> SNAADPEVCCFITKILCAHGGRMALDALLQEIALSEPQLCEVLQVAGPDRFVVLETGGEAGITRSVVATTRARVCRRKYCQRPCDNLHLCKLNLLGRCNYSQSERNLCKYSHEVLSEENFKVLKNHELSGLNKEELAVLLLQSDPFFMPEICKSYKGE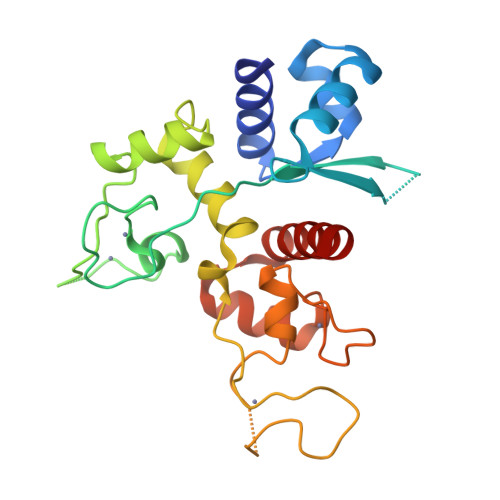GRQQICNQQPPCSRLHICDHFTRGNCRFPNCLRSHNLMDRKVLAIMREHGLNPDVVQNIQDICNSKHMQKN>[30x]MMIP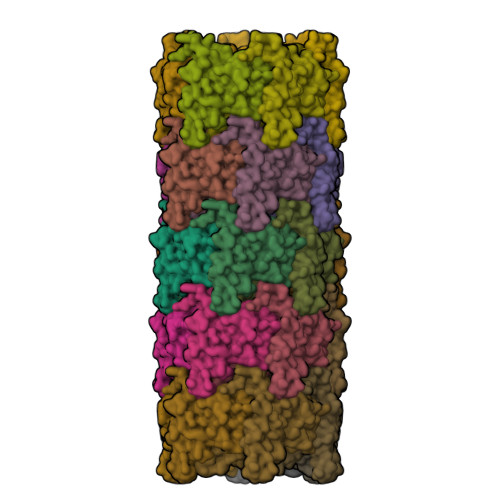QTLTNTNLFIDGVSFAGDVPSLTLPKLAVKTEQYRAGGMDAPVSIDMGLEAMEAKFSTNGARREALNFFGLADQSAFNGVFRGSFKGQKGASVPVVATLRGLLKEVDPGDWKAGEKAEFKYAVAVSYYKLEVDGREVYEIDPVNGVRAINGVDQLAGMRNDLGL>MQLAKVLGTVVSTSKTPNLTGVKLLLVQFLDTKGQPLERYEVAGDVVGAGLNEWVLVARGSAARKERGNGDRPLDAMVVGIIDTVNVASGSLYNKRDDGRLEAAAHHHHHH[10x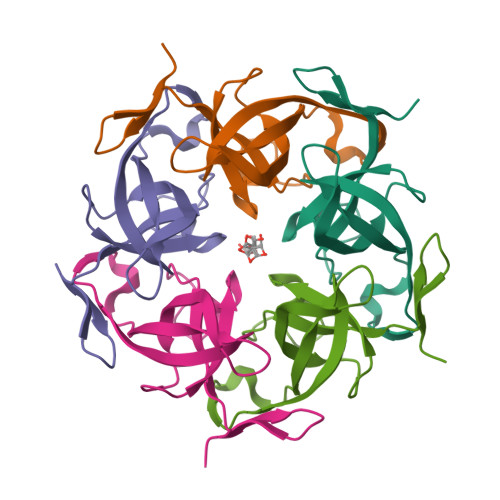]>[6x]MNESAGHNIKEDYFRVDMLLNKKGQVILYGPPGTGKTWIARKYVVEETNEKTPGNKWEFITFHQSYSYEEFIEGFRPRTDNEEKIRYVVEDGIFKKIALRALVKGLFELEDATIGKDKIHRLYILLTKKEPLSPTEYEEYLRLKRYLWELVGGLPKDKLKNLTPKFYLIIDEINRGNISKIFGELIT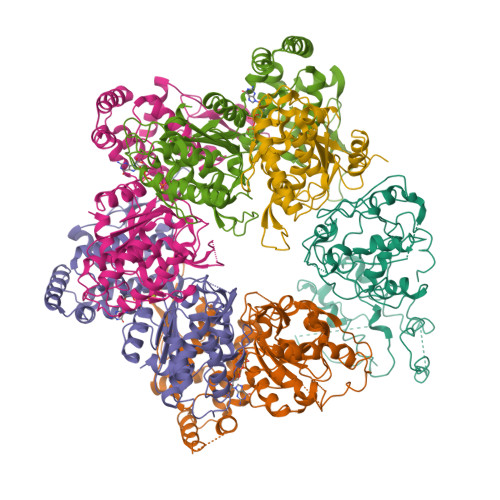LLEKDKRLGGENQLIVRLPYSGEPFAVPPNLYIIGTMNTADRSIALLDVALRRRFAFIEVEPRPEFLEKENLKKIREKKLKTEDRKRLNEKLNELFSKLGNDNYFLKTLLEKINVRITVVKDRDHRIGHSYFLNVETVEDLHHVWYYEVLPLLMEYFYNDWETIKWVLNEKGKEHGNVFFEKLRLTGPNGEEAYQLKVLEGDAFIGALKRIISKNTPSQEGGATTNEENSPENTQSQTEGD L-ALPHA-PHOSPHATIDYL-BETA-OLEOYL-GAMMA-PALMITOYL-PHOSPHATIDYLETHANOLAMINE 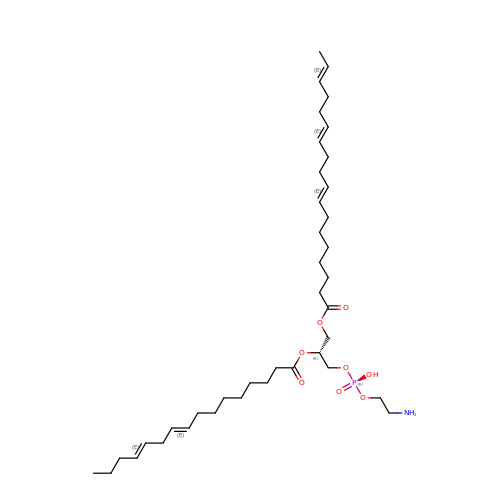| C39 H68 N O8 P | MABRTXOVHMDVAT-AAEGOEIASA-N> RILPEVKVEGELGGSVTIKCPLPEMHVRIYLCREMAGSGTCGTVVSTTNFIK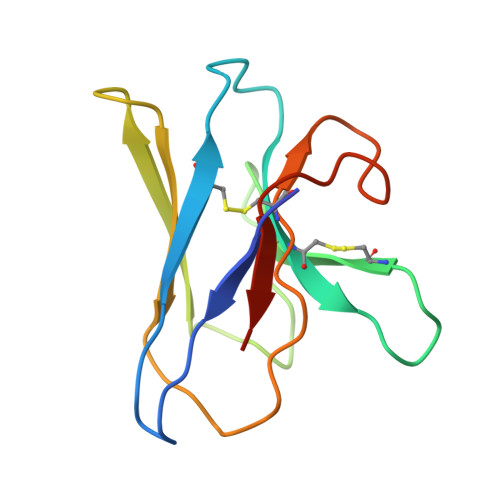AEYKGRVTLKQYPRKNLFLVEVTQLTESDSGVYACGAGMNTDRGKTQKVTLNVHS>PVDVSVSIFINKIYGVNTLEQTYKVDGYIVAQWTGKPRKTPGDKPLIVENTQIERWINNGLWVPALEFINVVGSPDTGNKRLMLFPDGRVIYNARFLGSFSNDMDFRLFPFDRQQFVLELEPFSYNNQQLRFSDIQVYTENIDNEEIDEWWIRGKASTHISDIRYDHLSSVQPNQNEFSRITVRIDAVRNPSYYLWSFILPLGLIIAASWSVFWLESFSERLQTSFTLMLTVVAYAFYTSNILPRLPYTTVIDQMIIAGYGSIFA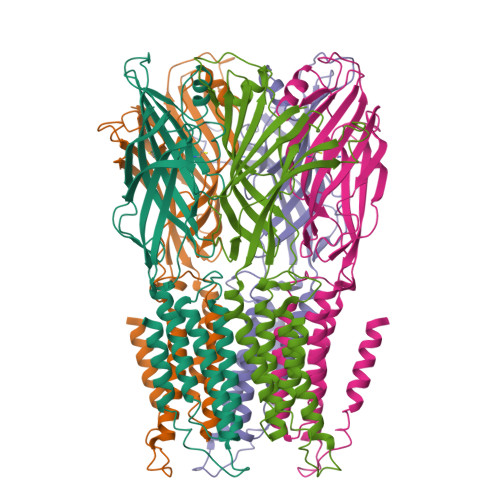AILLIIFAHHRQANGVEDDLLIQRCRLAFPLGFLAIGCVLVI[5x]KtrAB is a cation channel with a nucleotide-dependent RCK domain. The structure of the KtrAB complex revealed a homodimeric membrane protein (KtrB) assembled with a cytosolic RCK octameric ring, formed by the KtrA protein. KtrA binds nucleotides, ATP or ADP. ATP binding induces the adoption of a square-conformation by the octameric ring and increased K+ flux activity through KtrAB; ADP binding results in a non-square conformation and decreased flux.

As a control, we also analyzed the impact of mutating A80 since substitution with a bulkier side-chain was expected to cause a distortion of the nucleotide-binding site. As expected, A80P resulted in KtrAB inactivation. Crystal structures of the mutants that did not rescue the TK2420 growth phenotype (A80P and E125Q) reveal a different picture. The ATP-bound structures do not adopt a square conformation, displaying L1/L2 distances for A80P (at 3.9 Å resolution) of 52/23 Å and for E125Q (at 4.1 Å resolution and with two different half-rings in the asymmetric unit) of 34/30 Å and 42/27 Å. The ADP-bound structures are also non-square, showing ring conformations that are very similar to those observed with ATP: A80P (at 4.3 Å resolution) has L1/L2 distances of 52/22 Å and E125Q (at 4.0 Å resolution and with two rings) of 34/30 Å and 42/27 Å. In contrast, we found a large structural variability in the non-square structures, with four different conformational groups based on Cα N38 L1/L2 distances.

>[8x]MGRIKNKQFAVIGLGRFGGSICKELHRMGHEVLAVDINEEKVNAYASYATHAVIANATEENELLSLGIRNFEYVIVAIGPNIQASTLTTLLLKELDIPNIWVKAQNYYHHKVLEKIGADRIIHPEKDMGVKIAQSLSDENVLNYIDLSDEYSIVELLATRKLDSKSIIDLNVRAKYGCTILAIKHHGDICLSPAPEDIIREQDCLVIMGHKKDIKRFENEGM> MSKIEKLSILGVRSFGPHHPETIAFNTPLTLIVGYNGSGKTTVIECLKYATTGELPPNSTRNGAFIHDPDLVGEKEVRAQVKLSFRSTIGESYVVTRNIQLLVQRNNKRTQKTLEGSLLLRNNGERTVISTRVAELDKLVSEKLGVPPAILDAVIFCHQDDSLWPMSEPAALKKRFDEIFEAQKYTKVIENIRLLKKKKGDELKILKEREVQDKANKERAEKVDRLMAQLTREILEAREKCNELSKQMEEESAKIKDKYEQANSFLKIMNDLQTKTEKLEYKKDAIVELRSRIEELPDPDEVLRNTLDEYEQTINRIVADRDHKAAQFHDLQAELKSARDQHTAKAAEQGKHQSDKEKYERQLVARERMIREAAERHEIRGYNGDLDDRRIAIFNERIQKILNDKRRELERLQRENQEELDRKTAVIAERESRKQSVIRDRKAAKDRIISLGKDMASIQGELSSIDIDEGTEEMLRAEMKELQARIEAAKADEQNANLDAQIKEVNEEIWKLESLSAKLARELVECTRLASERAQLDLRRKQLAERKRELEIMTNTWNEQFSTLLGEGWRPETLERDFSDVLKQQQLLVGEHRKKKDATQQELKQAEYQLSNARNLHNKLTNEMEACMRAVQTAMKEARDLDSAPPVDEYITMLETDEKELAEVETALKLYDELKKHYSTIKDRALRFNKCYICDRDFTNQEAAKTRLLEKVAKRLGDEEKKELLEDQAAFMKSLDILRAVRVKYDTYQRLSSELPQLSREIDSETNRREDLVRRLEDQDLAFREADNKLQ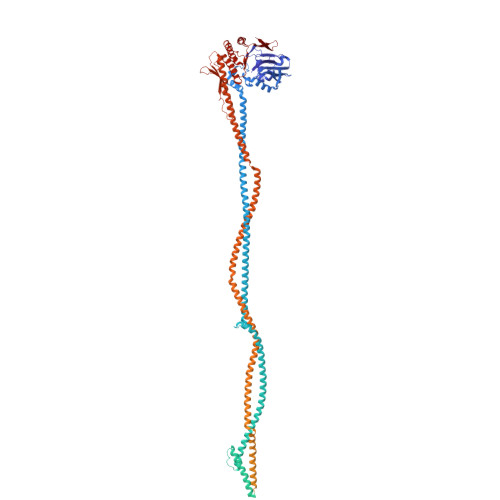EMETLNKHVMKITQLLKDISDAEKQVERSQQLSNIETRSADEINEEQTTCAEQTRAAQAKLTKLTAEKQRLKDLVRQLEVERLQLENKISSAVQQLERKKRLQESIARHKEDQNQARNAVQEADEELERLEPEIAGARAALDEARQACRAKEQKVAAERDAIAQTVSELNMINSEIQEYLDRGGPSSLAANQRAIANLETQMANLEGEMRELTVQINKLNKEIDNSDAKKRNIADNLTYRKNLREKDALEREIAELEARNAQEDYDRLIKEAHYLEAHRSKLNADRERLMGMMSTKDEEFRRLNEEYELDLKDAKAKYKETHIKVETTKAAIEDLGRGMAAVDHAIMQYHSKMMEQINRTIAELWQSTYQGTDIDTIQIRSDVESTTSSDSGTRRNYNYRVSMVKGDTEMDMRGRCSAGQKVLASIIIRLALAESFCANCGLIALDEPTTNLDSDNIRSLAESLHGIIKARQAQGNLQLIVITHDEEFLKYMQCSDFCDDFYRVKRDEKQNSVIVRESITRITE>MADDQGCIEEQGVEDSANEDSVDAKPDRSSFVPSLFSKKKKNVTMRSIKTTRDRVPTYQYNMNFEKLGKCIIINNKNFDKVTGMGVRNGTDKDAEALFKCFRSLGFDVIVYNDCSCAKMQDLLKKASEEDHTNAACFACILLSH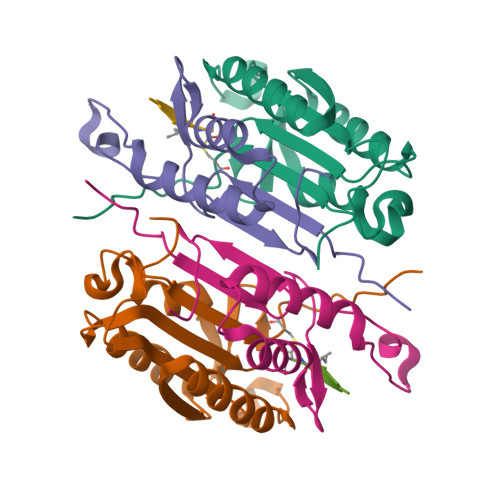GEENVIYGKDGVTPIKDLTAHFRGDRCKTLLEKPKLFFIQACRGTELDDGIQAD[2x];>[2x]SGPINDTDANPRYKIPVEADFLFAYSTVPGYYSWRSPGRGSWFVQALCSILEEHGKDLEIMQILTRVNDRVARHFESQSDDPHFHEKKQIPCVVSMLTKELYFSQLEHHHHHH>[2x]SMETVQLRNPPRRQLKKLDEDSLTKQPEEVFDVLEKLGEGSYGSVYKAIHKETGQIVAIKQVPVESDLQEIIKEISIMQQCDSPHVVKYYGSYFKNTDLWIVMEYCGAGSVSDIIRLRNKTLTEDEIATILQSTLKGLEYLHFMRKIHRDIKAGNILLNTEGHAKLADFGVAGQLTDTMAKRNTVIGTPFWMAPEVIQEIGYNCVADIWSLGITAIEMAEGKPPYA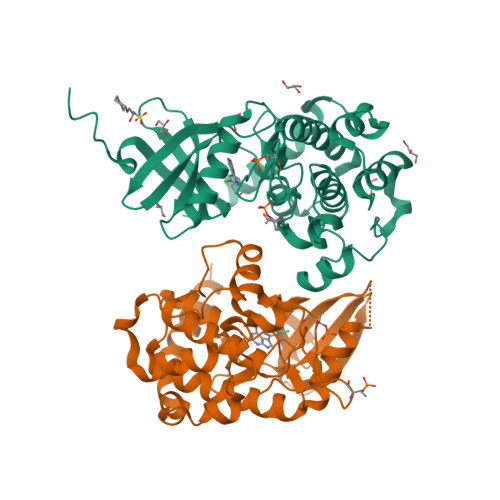DIHPMRAIFMIPTNPPPTFRKPELWSDNFTDFVKQCLVKSPEQRATATQLLQHPFVRSAKGVSILRDLINEAMDVKLKRQESQQREEG>[4x]GSAAKMAKNVDKPLFTATFNVQASSADYATFIAGIRNKLRNPAHFSHNRPVLPPVEPNVPPSRWFHVVLKASPTSAGLTLAIRADNIYLEGFKSSDGTWWELTPGLIPGATYVGFGGTYRDLLGDTDKLTNVALGRQQLADAVTALHGRTKADKPSGPKQQQAREAVTTLLLMVNEATRFQTVSGFVAGLLHPKAVAAASGKIGNEMKAQ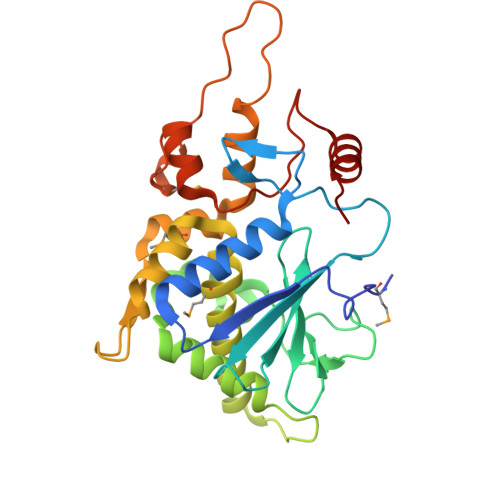VNGWQDLSAALLKTDVKPPPGKSPAKFAPIEKMGVRTAVQAANTLGILLFVEVPGGLTVAKALELFHASGGK> SNAAMLGGIEAGGTKFVCAVGREDGTIIDRIEFPTKMPDETIEKVIQYFSQFSLQAIGIGSFGPVDNDKTSQTYGTITATPKAGWRHYPFLQTVKNEMKIPVGFSTDVNAAALGEFLFGEAKGLDSCLYITIGTGIGAGAIVEGRLLQGLSHPEMGHIYIRRHPDDVYQGKCPYHGDCFEGLASGPAIEARWGKKAADLSDIAQVWELEGYYIAQALAQY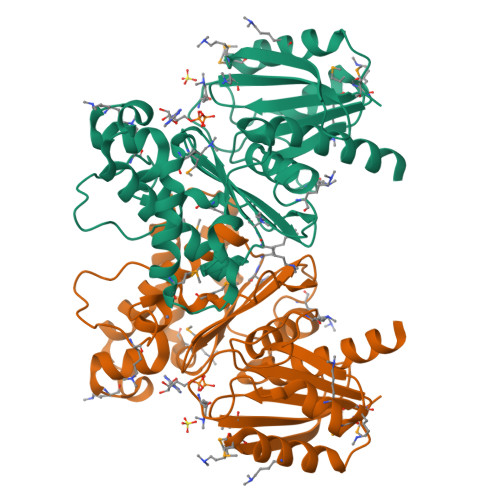ILILAPKKIILGGGVMQQKQVFSYIYQYVPKIMNSYLDFSELSDDISDYIVPPRLGSNAGIIGTLVLAHQALQAEAASGEVRS> APAVADKADNAFMMICTALVLFMTIP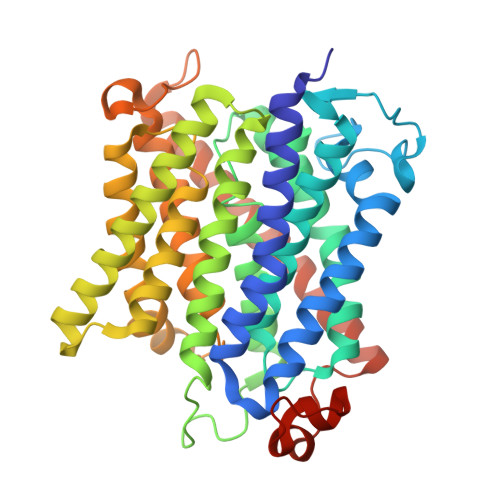GIALFYGGLIRGKNVLSMLTQVTVTFALVCILWVVYGYSLAFGEGNNFFGNINWLMLKNIELTAVMGSIYQYIHVAFQGSFACITVGLIVGALAERIRFSAVLIFVVVWLTLSYIPIAHMVWGGGLLASHGALDFAGGTVVHINAAIAGLVGAYLIGKRVGFGKEAFKPHNLPMVFTGTAILYIGWFGFNAGSAGTANEIAALAFVNTVVATAAAILGWIFGEWALRGKPSLLGACSGAIAGLVGVTPACGYIGVGGALIIGVVAGLAGLWGVTMLKRLLRVDDPCDVFGVHGVCGIVGCIMTGIFAASSLGGVGFAEGVTMGHQLLVQLESIAITIVWSGVVAFIGYKLADLTVGLRVPEEQEREGLDVNSHGENAYNAGTLVPR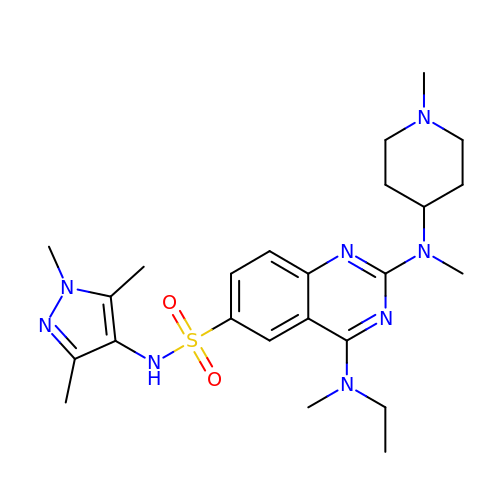4-[ethyl(methyl)amino]-2-[methyl-(1-methylpiperidin-4-yl)amino]-~{N}-(1,3,5-trimethylpyrazol-4-yl)quinazoline-6-sulfonamide | C24 H36 N8 O2 S | FKMXYCIDOKESEP-UHFFFAOYSA-N The proinflammatory cytokine tumor necrosis factor-alpha (TNFα) is a critical mediator of normal inflammatory responses but its overproduction can cause acute and chronic tissue damage. Here we have investigated the potential of macrocyclic peptides as another alternative class of TNF binders. Said system has allowed the discovery of M21, a high-affinity binder to TNFα capable of inducing dissociation of the trimeric state of the pro-inflammatory cytokine TNFα, a relevant clinical target, to an inactive dimeric form.

In order to better understand the effects of the M21 bicyclic peptide on TNFα structure and function we determined a structure of the peptide-cytokine complex by X-ray crystallography at 2.95 Å resolution. The asymmetric unit of the crystal consists of 2 copies of a TNFα—M21 bicycle complex at a ratio of 2 : 1. The structure shows the M21 peptide bound to a dimer of TNFα subunits (A and B) interacting with residues from both A and B and with an average interface area of TNFα and M21 of 231 Å2 (compared to 398 Å2 for the TNFα subunit interface). M21 is bound at a hydrophobic epitope adjacent but non-overlapping with the TNF (R1) receptor binding site but overlapping with the SPD304 binding site. The flat surface of the M21 bicycle formed by the organic core and W7 packs against the core of the A subunit involving H15, Y59 and Y151. The side-chains of the M21 loop 2 (residues L6, V9 and L10) make contacts with the B subunit. The only hydrogen bond observed between bicycle and TNFα (in both copies of the complex) is formed between amine group of W7 in loop2 and the hydroxyl group of Y119 side-chain in TNFα subunit B. No other intermolecular hydrogen bonds or salt bridges are observed, suggesting that the high-affinity interaction is largely driven by hydrophobic/van der Waals interactions and shape complementarity. The disassembly of TNFα trimers by M21 might occur either by induced TNFα trimer dissociation or by stabilization of a transient dimeric form. The latter is more consistent with the slow time-dependent effect of M21 action and with the inability of M21h to bind the stably trimeric transmembrane form of TNFα (tmTNF).

>VRSSSRTPSDKPVAHVVANPQAEGQLQWLNRRANALLANGVELRDNQLVVPSEGLYLIYSQVLFKGQGCPSTHVLLTHTISRIAVSYQTKVNLLSAIKSPCQRETPEGAEAKPWYEPIYLGGVFQLEKGDRLSAEINRPDYLDFAESGQVYFGIIAL[4x];>ACPPCLWQVLCG[2x]>GSHMVSVIKPEMKIKLCMRGTVNGHNFVIEGEGKGNPYEGTQILDLNVTEGAPLPFAYDILTTVFXNRAFTKYPADIQDYFKQTFPEGYHWERSMTYEDQGICTATSNISMRGDCFFYDIRFDGVNFPPNGPVMQKKTLKWEPSTEKMYVRDGVLKGDVNMALLLEGGGHYRCDFKTTYKAKKDV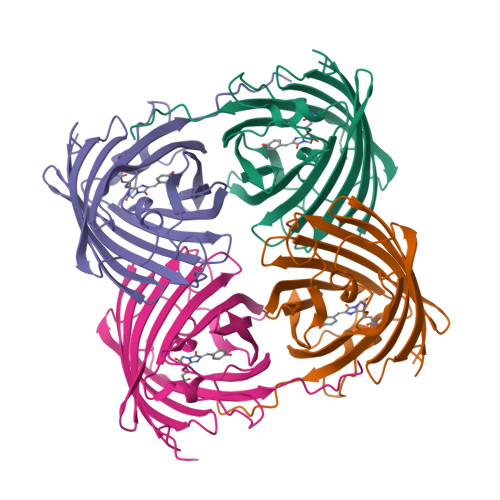RLPDYHFVDHRIEILKHDKDYNKVKLYENAVARYSMLPSQAK[4x]> MPSSSSEDAQGGNRFECVSNSTSPRRKNATKDEAACLQPRRSAVSGPREDVLCIRTTPQPHVRRGKSGPGRRKRMRFGR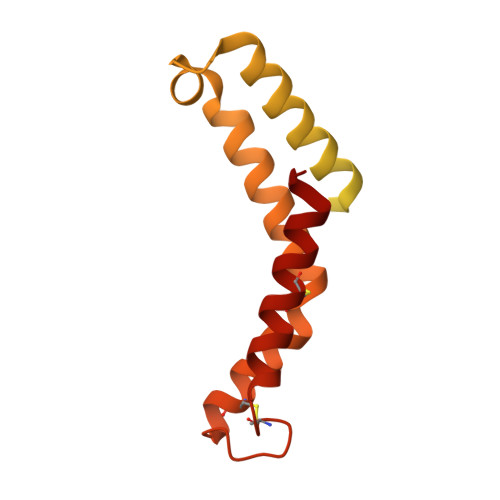ERERRDKKRGEGERKRTRFPFLRLHIEGGNANSRRPLCFPSRHSLLRNHYGSLSMAFRKVSPPKAPMSVFEARSSFLDLEQCARAAGPQRWEAECQGVRQRALQAAADVMSRECGAYGDSFFQCYRHGFRLEACQGEKATMQLLRCQRMVADRLVPL> MGNAVVVKKDFRIDLENELFIRGEVTLVEDQIKKPVLVISHGFRGYK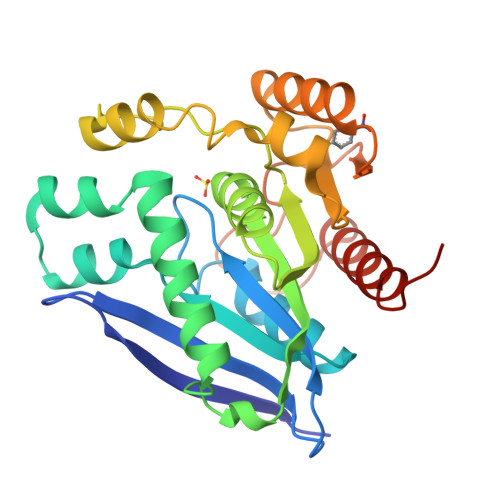DWGFWPYVAAWFAERGFYVVHFDFSRVGALNSGADEASVQKLSTVSRELSDLDAILSNLREHRLPLAEQAETERISLLGHSRAGGSNIIFAAEHSYIGSVIAWNGGPPPKAAAGNPNPFINDDVEHNKQRFDTARLLASLTAPVLIIQGGKDREALLEGQQLLKEAAPNQTYISIPDADHSFGGEHPFHHTTPYLEEALEVTHSFITKHYLEHHHHHH>MVRGFYLRFGEGVSEEANRRALALAEALLRAPPPGLLDAVPAYGVLYLEYDPRRLSRGRLLRLLKGLPQERAEEGRVVEIPVRYDGEDLPEVASRLGLSLEAVKALHQKPLYRVYALGFTPGFPFLAEVEPALRLPRKPHPRPRVPAHAVAVAGVQTGIYPLPSPGGWNLLGTSLVAVYDPHRETPFLLRPGDRVRFLEAEGPTPPEPRPLELLPEEPRLPALLVEEPGLMDLVVDGGRFLGGHLGLARSGPLDAPSARLANRLVGNGAGAPLLEFAYKGPVLTALRDLVAAFAGYGFVALLEGEEIPPGQSFLWPRGKTLRFRPRGPGVRGYLAVAGGLEVRPFLGSASPDLRGRIGRPLWAGDVLGLEALRPVRPGRAFPQRPLPEAFRLRLLPGPQFAGEAFRALCSGPFRVARADRVGVELLGPEVPGGEGLSEPTPLGGVQVPPSGRPLVLLADKGSLGGYAKPALVDPRDLWLLGQARPGVEI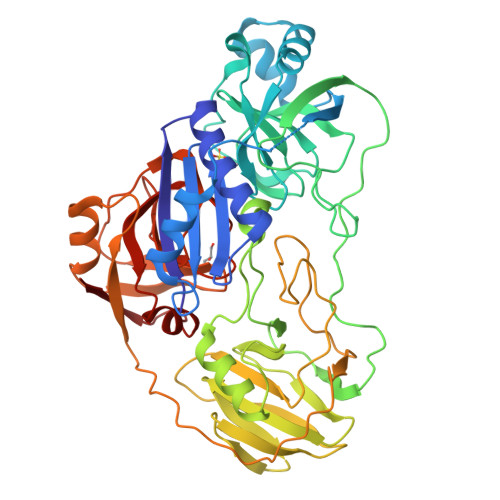HFTSG[3x]ETHYL 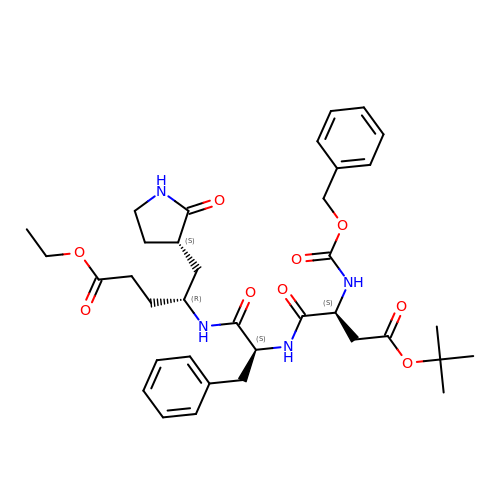(5S,8S,11R)-8-BENZYL-5-(2-TERT-BUTOXY-2-OXOETHYL)-3,6,9-TRIOXO-11-{[(3S)-2-OXOPYRROLIDIN-3-YL]METHYL}-1-PHENYL-2-OXA-4,7,10-TRIAZATETRADECAN-14-OATE | C36 H48 N4 O9 | DAQSBCFYXOITIO-CRNKYVSFSA-N> SADAQSFLNRVCGVSAARLTPCGTGTSTDVVYRAFDIYNDKVAGFAKFLKTNCCRFQEKDEDDNLIDSYFVVKRHTFSNYQHEETIYNLLKDCPAVAKHDFFKFRIDGDMVPHISRQRLTKYTMADLVYALRHFDEGNCDTLKEILVTYNCCDDDYFNKKDWYDFVENPDILRVYANLGERVRQALLKTVQFCDAMRNAGIVGVLTLDNQDLNGNWYDFGDFIQTTPGSGVPVVDSYYSLLMPILTLTRALTAESHVDTDLTKPYIKWDLLKYDFTEERLKLFDRYFKYWDQTYHPNCVNCLDDRCILHCANFNVLFSTVFPPTSFGPLVRKIFVDGVPFVVSTGYHFRELGVVHNQDVNLHSSRLSFKELLVYAADPAMHAASGNLLLDKRTTCFSVAALTNNVAFQTVKPGNFNKDFYDFAVSKGFFKEGSSVELKHFFFAQDGNAAISDYDYYRYNLPTMCDIRQLLFVVEVVDKYFDCYDGGCI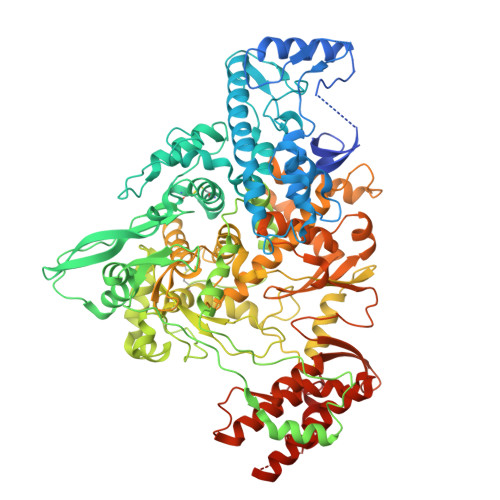NANQVIVNNLDKSAGFPFNKWGKARLYYDSMSYEDQDALFAYTKRNVIPTITQMNLKYAISAKNRARTVAGVSICSTMTNRQFHQKLLKSIAATRGATVVIGTSKFYGGWHNMLKTVYSDVENPHLMGWDYPKCDRAMPNMLRIMASLVLARKHTTCCSLSHRFYRLANECAQVLSEMVMCGGSLYVKPGGTSSGDATTAYANSVFNICQAVTANVNALLSTDGNKIADKYVRNLQHRLYECLYRNRDVDTDFVNEFYAYLRKHFSMMILSDDAVVCFNSTYASQGLVASIKNFKSVLYYQNNVFMSEAKCWTETDLTKGPHEFCSQHTMLVKQGDDYVYLPYPDPSRILGAGCFVDDIVKTDGTLMIERFVSLAIDAYPLTKHPNQEYADVFHLYLQYIRKLHDELTGHMLDMYSVMLTNDNTSRYWEPEFYEAMYTPHTVLQ>[16x]ASWSHPQFEKIEGRRDRGPEFMAKQYKNLVNGEWKLSENEITIYAPATGEELGSVPAMTQAEVDAVYASAKKALSDWRTLSYVERAAYLHKAADILVRDAEKIGAILSKEVAKGHKAAVSEVIRTAEIINYAA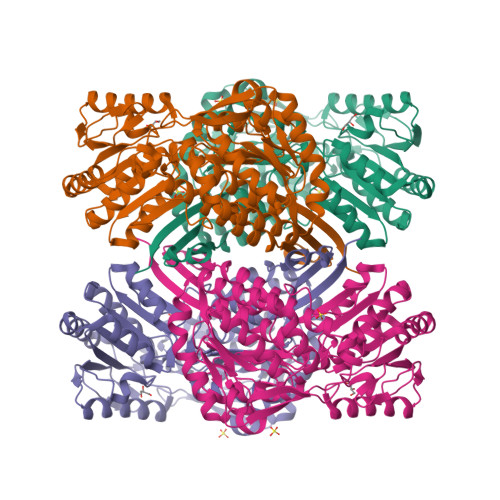EEGLRMEGEVLEGGSFEAASKKKIAIVRREPVGLVLAISPFNYPVNLAGSKIAPALIAGNVVALKPPTQGSISGLLLAEAFAEAGIPAGVFNTITGRGSVIGDYIVEHEAVNFINFTGSTPIGEGIGKLAGMRPIMLELGGKDSAIVLEDADLALAAKNIVAGAFGYSGQRSTAVKRVLVMDKVADQLAAEIKTLVEKLSVGMPEDDADITPLIDTSAADFVEGLIKDATDKGATALTAFNREGNLISPVLFDHVTTDMRLAWEEPFGPVLPIIRVTTVEEAIKISNESEYGLQASIFTTNFPKAFGIAEQLEVGTVHLNNKTQRGTDNFPFLGAKKSGAGVQGVKYSIEAMTTVKSVVFDIQ Podophages that infect gram-negative bacteria, such as Pectobacterium pathogen ΦM1, encode tail assemblies too short to extend across the complex gram-negative cell wall. To overcome this, podophages encode a large protein complex (ejectosome) packaged inside the viral capsid and correspondingly ejected during infection to form a transient channel that spans the periplasmic space. Here, we report a near-complete atomic model of the bacteriophage ΦM1.

Using cryo-EM, we investigated the whole particle structure of bacteriophage ΦM1, identifying two decorations with relatively uncommon morphology, and a tail fiber/spike assembly with features similar to the recently published structure of Shigella phage HRP29 and phage T7. An adaptor assembly (gp52) interfaces with the portal and six tail fibers (trimeric gp47), each of which appears composed of long helical bundles much like phage T7, as well as adapts trimers of spike protein (gp39) which may be homologous to those in phage P22, another podophage, and 9NA, a siphovirus. Gp39 was poorly ordered in our reconstructions and was not modeled. However, AlphaFold2 multimer predicts a structure similar to phage HRP29 gp52. The short tail assembly has the closest similarity to bacteriophage HRP29 (16). The core consists of tetrameric and octameric ejection proteins which form a ∼1.5-MDa ejectosome that must transition through the ∼30 Å aperture created by the short tail nozzle assembly that acts as the conduit for the passage of DNA during infection.

>MAFDGSIKSLLQGVSQQVPRERLDGQVSVQLNRLSDVVNGNRRRPGARYLADVPTTSQYDDHVFASYVDVQDTANHVIINTETGQLLVISEDFSTTLHNSTQQYLVASAASAIQTATLRGDLYIANTEKAPTKVFGSTTQQDPTKAGFYFVRTPALQKDYDITLSNSTGTYTYTYRTPTGTGTGDADLAKPSYIISDLLAKINAQTGTHGITATAYDAYMFLSSNTVSLSVTTNAGSTYATGSNQSRVSVVSDLPARLPAVGNGASVAVGTTERNFVWYQYDSATSVWKEAGAYGSPTGFSNMPIRISLDGVYTVETPAYEGRLAGSDETNEDPGFIDNGVTGFGAYQGRLVILAGPEVCMSAAGNPLRWYRSTVTALLTDDPINIFSGAATSTNFRHCVQFNKDLLLFARSCQAVVPSSNAAITPQTAQIVITSGYTTDTLAQPGVVGRSVLYSMPRTEHFAGVLEIIPSNTTDSQYTSNDITAHIPRYLPGRIRSIVSSTTSNSSAFICTGDSRSLFIQDYLWSGDEKVQSAWHQWTLPYPIVCTWFVRDRVYIGMRDGTTILVVTIEPQAGNTIDSYVRPFSDVYLRVTITDRQFALPTRLRAAVGSGEGLFITFADTSMGGMWVGYESIDPTTYVVTTVRNVPDGEYFVGLRYTSVLSPTPPLVRDANGIVIGTYQSLLVRYELTLKDSGEFHAIITDSSRTLTDGNYSSLVYSSTELLPNNPTDASLGRTIIPVRAQAQDTVATFEANADTDLCILDIEYVLQYRARRKRI[6x];>MYSVQIAVSDGTLTRIALSIEYFEKDDITLYRNLELTPLVLGTDWQWDGDTHINLLTGIPVPVGSYITVRRNTDIDRAFNIYDGGAAFNRETLDENFKQMIYLAQEFTEGNGLTGLYFPLDMHGFQIKNLGEPTDPGDAVTKQYVDTANTAQNANFNASQQAQDQAVAASQAVQDNRLASLENTFVQATSSYPWYTVSTSTTDTFTPGFNFTKAAVYINGVCQTPDYSYIVVANQILLADPVPLGTMVFARLGEDIQNDDDFATTAQLSAVQANLQDEIDVTNTEVSNKASKGANSDISSLSGLTTPLSAAQGGTGNNTGNAATATVLATPRTIQTNLASTSAASFNGSANITPGVTGNLPVTNGGTGAGSAPSARANLGAAMNGINNDISNLAALTGGITGLTTGTAAASGIVGEVASAASSSATNLVSGSVINIISLSLPAGDWELESAFQIINTGNVTALAFGVSTTTGVLPTPWYDVYSITTTIGSGTSNRQGMARRVLLSTTTTVYLVAQATFTGTATANGYVRARRVR[18x]> MMNAQKSKIALLLAASAVTMALTGCGGSDGNNGNDGSDGGEPAGSIQTLNLDITKVSYENGAPMVTVFATNEADMPVIGLANLEIKKALQLIPEGATGPGNSANWQGLGSSKSYVDNKNGSYTFKFDAFDSNKVFNAQLTQRFNVVSAAGKLADGTTVPVAEMVEDFDGQGNAPQYTKNIVSHEVCASCHVEGEKIYHQATEVETCISCHTQEFADGRGKPHVAFSHLIHNVHNANKAWGKDNKIPTVAQNIVQDNCQVCHVESDMLTEAKNWSRIPTMEVCSSCHVDIDFAAGKGHSQQLDNSNCIACHNSDWTAELHTAKTTATKNLINQYGIETTSTINTETKAATISVQVVDANGTAVDLKTILPKVQRLEIITNVGPNNATLGYSGKDSIFAIKNGALDPKATINDAGKLVYTTTKDLKLGQNGADSDTAFSFVGWSMCSSEGKFVDCADPAFDGVDVTKYTGMKADLAFATLSGKAPSTRHVDSVNMTACANCHTAEFEIHKGKQHAGFVMTEQLSHTQDANGKAIVGLDACVTCHTPDGTYSFANRGALELKLMKKHV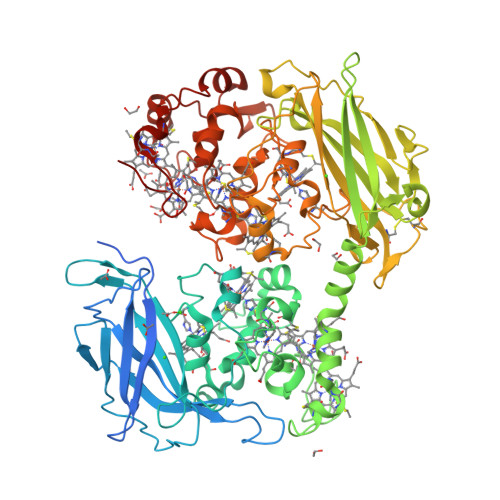EDAYGLIGGNCASCHSDFNLESFKKKGALNTAAAADKTGLYSTPITATCTTCHTVGSQYMVHTKETLESFGAVVDGTKDDATSAAQSETCFYCHTPTVADHTKVKM>[2x]MSELFSERIPPQSIEAEQAVLGAVFLDPAALVPASEILIPEDFYRAAHQKIFHAMLRVADRGEPVDLVTVTAELAASEQLEEIGGVSYLSELADAVPTAANVEYYARIVEEKSVLRRLIRTATSIAQDGYTREDEIDVLLDEADRKIMEVSQRKHSGAFKNIKDILVQTYDNIEMLHNRDGEITGIPTGFTELDRMTSGFQRSDLIIVAARPSVGKTAFALNIAQNVATKTNENVAIFSLEMSAQQLVMRMLCAEGNINAQNLRTGKLTPEDWGKLTMAMGSLSNAGIYIDDTPSIRVSDIRAKCRRLKQESGLGMIVIDYLQLIQGSGRSKENRQQEVSEISRSLKALARELEVPVIALSQLSRSVEQRQDKRPMMSDIRESGSIEQDADIVAFLYRDDYYNKDSENKNIIEIIIAKQRNGPVGTVQLAFIKEYNKFVNLERRFDEAQIPPGA;> KLLPAFQNAERLLLAHMMRSRDVALVVQE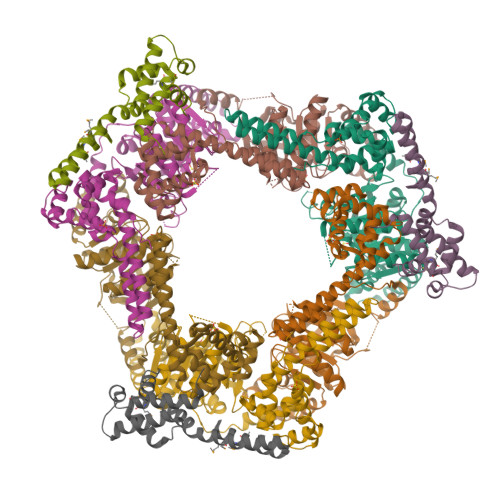RIGGRFNIEEHRALAAYIYAFYEEGHEADPGALISRIPGELQPLASELSLLLIADDVSEQELEDYIRHVLNRPKWLMLKVKEQEKTEAERRKDFLTAARIAKEMIEMKKMLSSS>MPVAHVALPVPLPRTFDYLLPEGMTVKAGCRVRVPFGKQQERIGIVVSVSDASELPLNELKAVVEVLDSEPVFTHSVWRLLLWAAD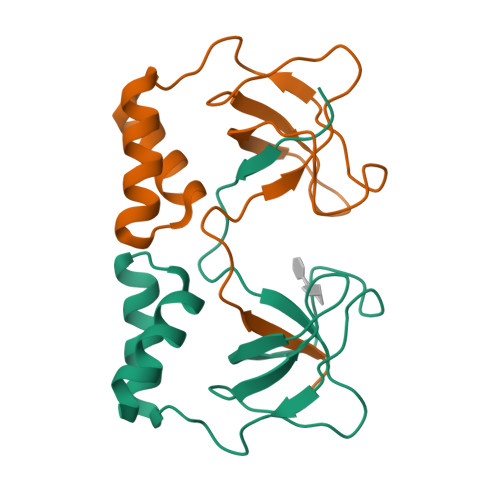YYHHPIGDVLFHALPILLR[4x]> MAATAAEAVASGSGEPREEAGALGPAWDESQLRSYSFPTRPIPRLSQSDPRAEELIENEEPVVLTDTNLVYPALKWDLEYLQENIGNGDFSVYSASTHKFLYYDEKKMANFQNFKPRSNREEMKFHEFVE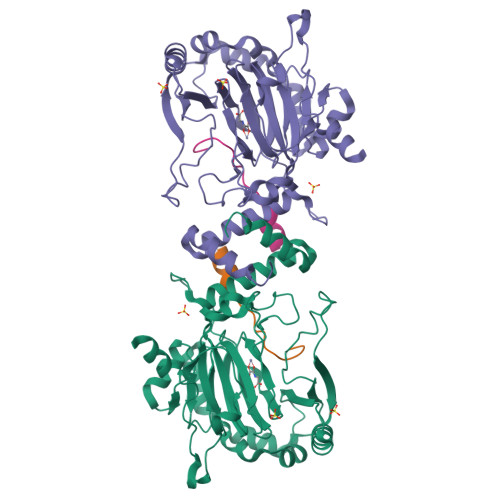KLQDIQQRGGEERLYLQQTLNDTVGRKIVMDFLGFNWNWINKQQGKRGWGQLTSNLLLIGMEGNVTPAHYDEQQNFFAQIKGYKRCILFPPDQFECLYPYPVHHPCDRHSQVDFDNPDYERFPNFQNVVGYETVVGPGDVLYIPMYWWHHIESLLNGGITITVNFWYKGAPTPKRIEYPLKAHQKVAIMRNIEKMLGEALGNPQEVGPLLNTMIKGRYN;> HLEVVKLLLEHGADVDAQDK> MDETGKELVLALYDYQEKSPRE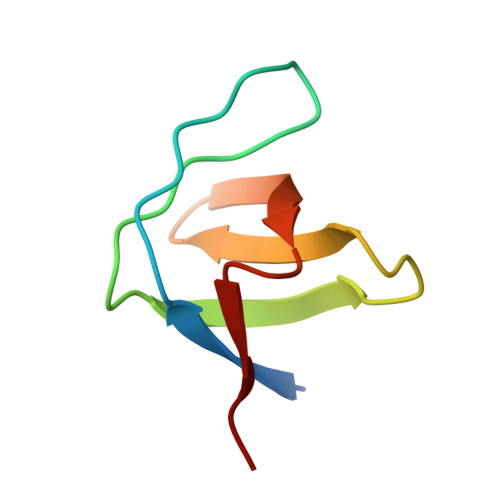VTMKKGDILTLLNSTNKDWWKVEVNDRQGFVPAAYVKKLD>[2x]GLEPVRRRPGMYTDTTRPNHLGQEVIDNSVDEALAGHAKRVDVILHADQSLEVIDDGRGMPVDIHPEEGVPAVELILCRLHA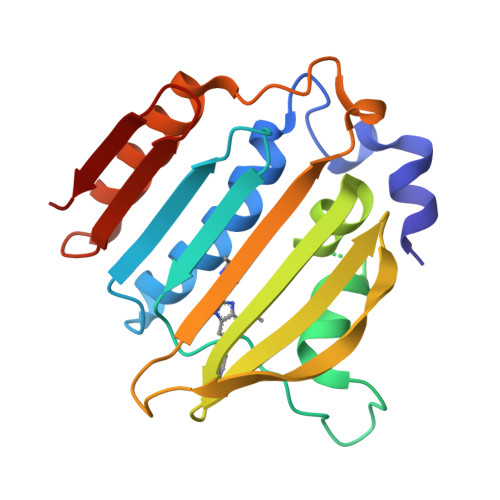GGKFSNKNYQFSGGLHGVGISVVNALSKRVEVNVRRDGQVYNIAFENGEKVQDLQVVGTCGKRNTGTSVHFWPDETFFDSPRFSVSRLTHVLKAKAVLCPGVEITFKDEINNTEQRWCY> DRRHVLLQAEFYQRSEGPDKAWAQFGFHFDADELFHVELDAAQTVWRLPEFGRFASFEAQGALQNMAVGKQNLEVMISNSNRSQQDFVTPELALFPAEAVSLEEPNVLICYADKFWPPVATMEWRRNGAVVSEGVYDSVYYGRPDLLFRKFSYLPFVPQRGDVYSCAVRHWGAEGPVQRMWEPE;> KMSMSTMNMPMAMKVGGGGSGGGGSGGGGSSAFFFCGAIFECHYLNGTERVRYLQRYIYNRQQLVHFDSDVGKFVADTPLGEPQAEYWNSNAELLENIMNIADGSCRHNYGILESFTVQRSVEPKVRVSALQSGSLPETDRLACYVTGFYPPEIEVKWFLNG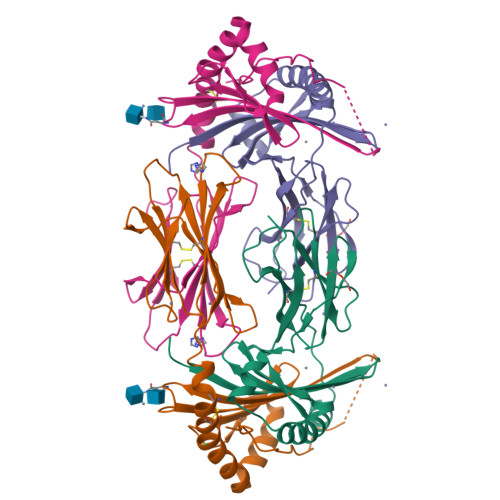REETERVVSTDVMQNGDWTYQVLVVLETVPRRGDSYVCRVEHASLRQPISQAWEPPADAGRSK In addition, the molecular interplay of the surface-exposed TlpA (renamed Etrx1) with its extracellular paralogue Etrx2 on oxidative stress resistance and virulence are unknown. This study discovers the unique molecular architecture of two surface-exposed thioredoxin-systems, Etrx1 and Etrx2 and their redox partners CcdA1, CcdA2 and SpMsrAB2 as important pneumococcal extracellular reducing systems essential for pneumococcal pathogenesis and oxidative stress resistance. The bioinformatic analysis of pneumococcal genomes identified two genes encoding surface-exposed thioredoxin-like lipoproteins, renamed here Etrx1 and Etrx2. According to the accepted catalytic mechanism of thioredoxin-like proteins, Etrx1/Etrx2 would bind their redox partner SpMsrAB2 by means of a hydrophobic surface and subsequently perform a nucleophilic attack on the target disulphide bond via the N-terminal nucleophilic thiolate of the CXXC motif (Cys84 in Etrx1, Cys81 in Etrx2). Surface-exposed Etrx1 and Etrx2 deliver electrons to the SpMsrAB2 protein for the reduction of MsrA2 (by Etrx1 or Etrx2) and MsrB2 (by Etrx2) domains.

Attempts to obtain the reduced form of Etrx2 by co-crystallization with β-mercaptoethanol resulted in a new oxidized structure in which Etrx2 forms a complex with a 2-hydroxyethyl disulfide (HED) molecule. A different conformation of the β4–α3 loop was observed coupled with the presence of the HED molecule at the hydrophobic cavity. Etrx2 has an unprecedented hydrophobic cavity close to the active site. The presence of a hydrophobic patch near the active site has been associated with substrate recognition in other TDORs. In the structure of the oxidized forms of Etrx2, a detergent molecule (Cyclofos-3™) or a HED molecule is bound to this hydrophobic pocket, very likely mimicking the redox partner interaction. The CXXC motif (81CGPC84) defines the active site. Many thioredoxin-like proteins share also a proline residue within the CXXC motif. This proline residue is also present in the CXXC motif of Etrx2, but not in Etrx1. The Etrx2 binding site presents a hydrophobic character while Etrx1 presents a highly basic character in this region.

>[2x]MGSSHHHHHHMSGENLYFQGASGEEETKKTQAAQQPKQQTTVQQIAVGKDAPDFTLQSMDGKEVKLSDFKGKKVYLKFWASWCGPCKKSMPELMELAAKPDRDFEILTVIAPGIQGEKTVEQFPQWFQEQGYKDIPVLYDTKATTFQAYQIRSIPTEYLIDSQGKIGKIQFGAISNADAEAAFKEMN> AKPFELLVSFLNTPKYGTFDPTPVVPVFFPFWFGMIVGDIGYALLFYLVGRWLSGYVKRNEPLVIDLFALKLKPQVIGKLVHILNWMVFWTVVWGVIYGEFFGTFLEHLGVFGTPEHPGLIPILIHRIDTAKTANLLILLSVAF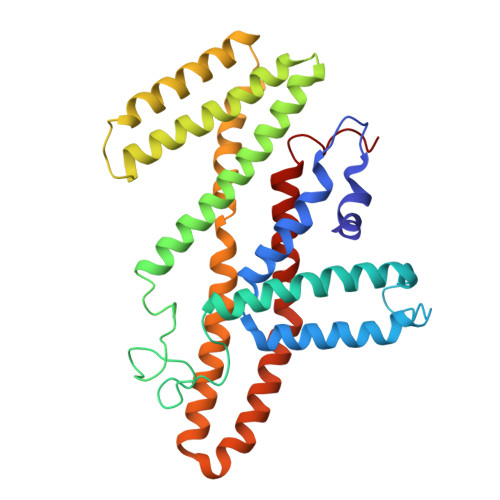GVVLVFFGLALRAYLGLKHRHMAHFWEGVGYLGGLVGVLALAASYLGNLQAGWLQGLMYLGFGVFLLAVLMSRIWLMIPEIFTQAGHILSHIRIYAVGAAGGILAGLLTDVGFALAERLGLLGVLLGLLVAGVLHLLILLLTTLGHMLQPIRLLWVEFFTKFGFYEENG>[2x]APAPTVNTHFGKLRGARVPLPSEILGPVDQYLGVPYAAPPIGEKRFLPPEPPPSWSGIRNATHFPPVCPQNIHTAVPEVMLPVWFTANLDIVATYIQEPNEDCLYLNVYVPTEDGSGAKKQGEDLADNDGDEDEDIRDSGAKPVMVYIHGGSYMEGTGNMIDGSVLASYGNVIVITLNYRVGVLGFLSTGDQAAKGNYGLLDQIQALRWVSENIAFFGGDPRRITVFGSGIGASCVSLLTLSHHSEGLFQRAIIQSGSALSSWAVNYQPVKYTSLLADKVGCNVLDTVDMVDCLRQKSAKELVEQDIQPARYHVAFGPVIDGDVIPDDPEILMEQGEFLNYDIMLGVNQGEGLKFVEGVVDPEDGVSGTDFDYSVSNFVDNLYGYPEGKDTLRETIKFMYTDWADRDNPETRRKTLVALFTDHQWVEPSVVTADLHARYGSPTYFY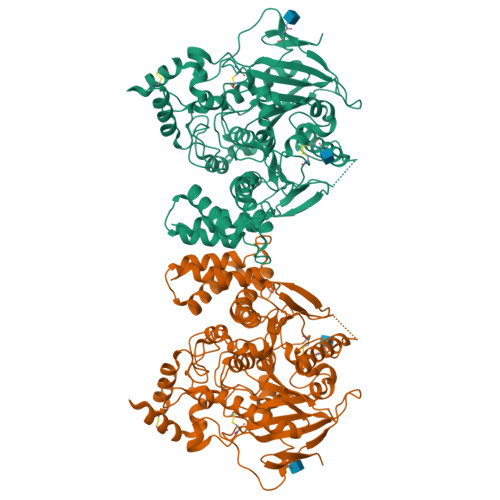AFYHHCQSLMKPAWSDAAHGDEVPYVFGVPMVGPTDLFPCNFSKNDVMLSAVVMTYWTNFAKTGDPNKPVPQDTKFIHTKANRFEEVAWSKYNPRDQLYLHIGLKPRVRDHYRATKVAFWKHLVPHLYNLHDMFHYTSTTTKVPPPDTTHSSHITRRPNGKTWSTKRPAISPAYSNENAPGSWNGDQDAGPLLVENPRDYSTEHHHHHH> GHTSGTYNDSLLTINSDYDAYLLDFPLMGDDFMLYLARMEL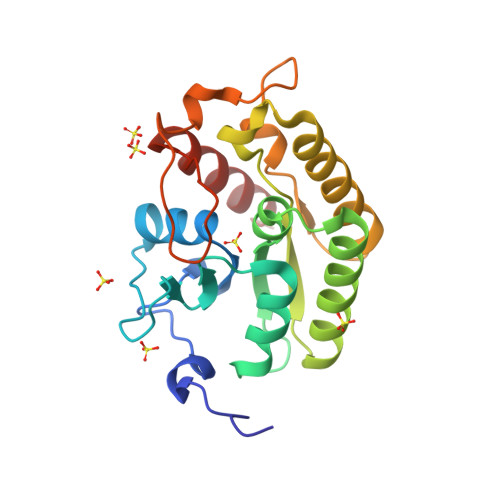KCRFRRHERVLQSGLCVSGLTINGARNRLKRVQLPEGTQIIVNIGSVDIMRGKPLVQIEHDFRLLIKEMHNMRLVPILTNLAPLGNYCHDKVLCDKIYRFNKFIRSECCHLKVIDIHSCLINERGVVRFDCFQASPRQVTGSKEPYLFWNKIGRQRVLQVIETSLEY> MYLTLQE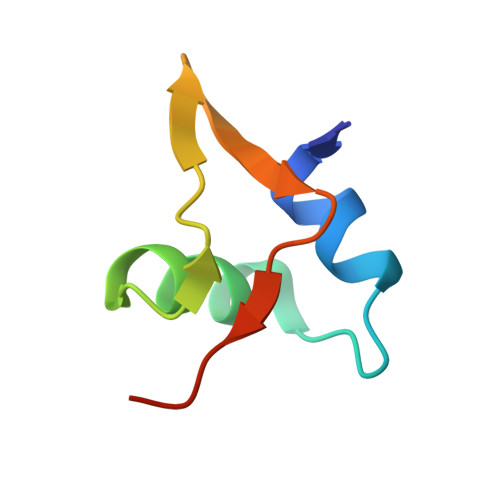WNARQRRPRSLETVRRWVRESRIFPPPVKDGREYLFHESAVKVDLNRP> GPLGSRQDKMREEGLQLVSMIREGEAAGACPEEIFSALQYSGTEVPLQWLRSELPYVLEMVAELAGQQDPGLGAFSCQEARRAWLDRHGNLDEA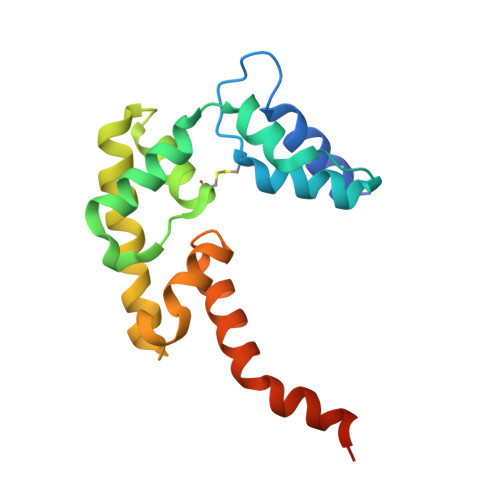VEECVRTRRRKVQELQSLGFGPEEGSLQALFQHGGDVSRALTELQRQRLEPFRQRLWDSGPEPTPSWD>[2x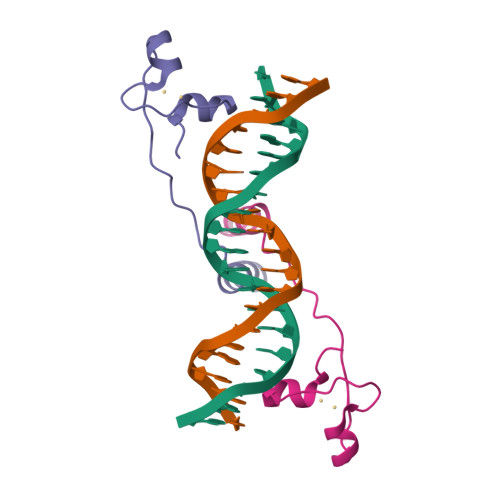]MKLLSSIEQACDICRLKKLKCSKEKPKCAKCLKNNWECRYSPKTKRSPLTRAHLTEVESRLERLEF In particular, one intensely studied protein, Legionella effector DrrA (Defect in Rab1 recruitment A, also referred to as SidM, substrate of Icm/Dot), is secreted early during infection, and it manipulates the vesicular trafficking regulator Rab1 (Ras-related protein Rab-1). DrrA consists of three functional domains. The N-terminal domain possesses AMPylation activity (also referred to as adenylylation). AMPylation is a post-translational modification (PTM) in which an adenosine triphosphate (ATP) is utilised in order to transfer adenosine monophosphate (AMP) to hydroxyl-bearing amino acid side chains.

Therefore, we also generated the TReND-1-linked complex with the GTPase domain of the close Rab1b-homologue Rab8a (amino acids 6−176; Rab8a6-176). In order to obtain insight into the molecular basis of DrrA substrate recognition, we determined the crystal structure of the DrrA16-352:TReND-1:Rab8a6-176 complex bound to GppNHp at 2.1 Å resolution (DrrA16-352:TReND-1:Rab8a6-176 will be referred to as DrrA:Rab8a hereafter for clarity). The complex binding mode observed in the crystal structure was unexpected since the Rab molecule does not interact with the catalytic centre of DrrA16-352 constituted by the catalytically important residues D110DrrA and D112DrrA13. Instead, Rab8a:GppNHp binds to a surface patch opposite the catalytic centre that we refer to as the non-conventional (NC) Rab binding site (RBS), hereafter referred to as NC-RBS. In the DrrA:Rab8a complex structure, switch I (E30Rab8a, F33Rab8a and N34Rab8a), the interswitch region (D44Rab8a and K58Rab8a), and switch II (Q60Rab8a and R69Rab8a) of Rab8a mainly interact with the N-terminal half of the ATPase domain of DrrA opposite the catalytic motif, centred at amino acids R70DrrA, Q71DrrA and K74DrrA. Based on the structures of other ATases belonging to the DNA polymerase β-like enzyme family, the catalytic motif of DrrA is expected to be G98-S99-L100-X11-D110-X-D112DrrA, with D110DrrA and D112DrrA involved in coordinating the essential magnesium ion. In contrast to the previous DrrA8-218 fragment structure, the position of D110DrrA and D112DrrA is well defined and the residues appear to be capable of Mg2+ coordination. The covalently bound TReND-1 is well defined in the electron density in the complex crystal structure. The structure of free Rab8a:GppNHp superimposes very well with Rab8a in the NC-RBS-complex, with an RMSD of 0.38 Å, indicating that binding of Rab8a to DrrA does not result in global structural changes in Rab8a. Indeed, upon Rab binding, helix α3 may be pulled into the protein core, and D110DrrA (β2), D112DrrA (β2) and D150DrrA (α4−α5 loop) move together so that the active Mg2+ coordinating function of these amino acid residues can be fulfilled.

> SHMDYLFKLLLIGDSGVGKTCVLFRFSEDAFNSTFISTIGIDFKIRTIELDGKRIKLQIWDTAGQERFRTITTAYYRGAMGIMLVYDITNEKSFDNIRNWIRNIEEHASADVEKMILGNKCDVNDKRQVSKERGEKLALDYGIKFMETSAKANINVENAFFTLARDIKAKMDKK;> GHMFGSLYSDERDKPLLSPTAQKKFEEYQNKLANLSKIIRENEGNEVSPWQEWENGLRQIYKEMIYDAFDALGVEMPKDMEVHFAGSLAKAQATEYSDLDAFVIVKNDEDIKKVKPVFDALNNLCQRIFTASNQIYPDPIGINPSRLIGTPDDLFGMLKDGMVADVEATAMSILTSKPVLPRYECGEELRDKIKQEPSFSNMVSAKKFYNKAIKDFTAPKEGAEVVSVKTHIMRPIDFMLMGLREEFNLYSEDGAHLSAPGTIRLLREKNLLPEEQIARIESVYNQAMSKRFELHAEHKKEHDEMPYSDAKAMLDEVAKIRELGVQRVTRIENLENAKKL>MWDTSKDYRLLVAEKSVELFIRTIEGAKFRGQWDKKRSIQLAKEMIPDIQALRYSYIDPEELVDTPQMKDLKEKAKGIIEALGGEDWHHKFLSQASREDREKVEEQVARIKFFLNTILNLDRRLKLGKINDPVIAVDIVVGEVMSVGKHPSADRL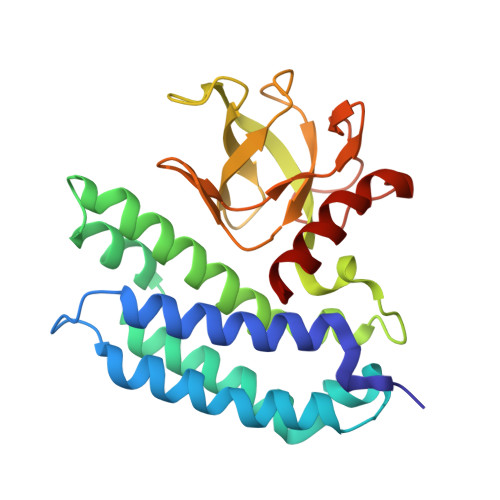LVTNVNIGERAVTVVTNDLTVKEGNRVAVALLPPRNFFGIVSEGMFLGAGEGVLKNVKGEIGGLPKGIPLEALNETRNAVEAFLKG[2x]>MKKIGIIGGTTPESTLYYYKKYIEISREKFEKYFYPELIIYSINFKEFFQNPEGWEGRKKILINAAKALERAGAELIAFAANTPHLVFDDVQREVNVPMVSIIDAVAEEILKRGVRKVLLLGTKTTMTADFYIKTLEEKGLEVVVPNDEEKEELNRIIFEELAFGNLKNKEWIVRLIEKYRESEGIEGVILGCTELPLAIKQGDVSVEVFDSAEIHMRKLIEL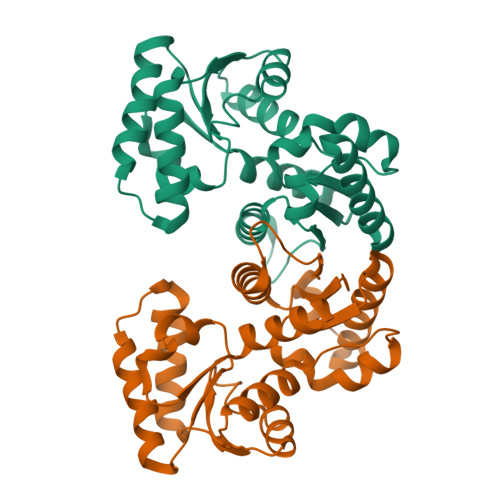ASE[2x]3,5-bis(fluoranyl)-~{N}-[3-[(4-methoxyphenyl)sulfamoyl]phenyl]benzamide 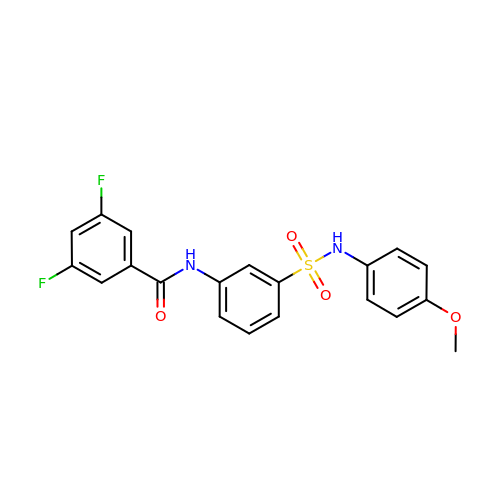| C20 H16 F2 N2 O4 S | PHNKXJVGPMJTLZ-UHFFFAOYSA-N> SA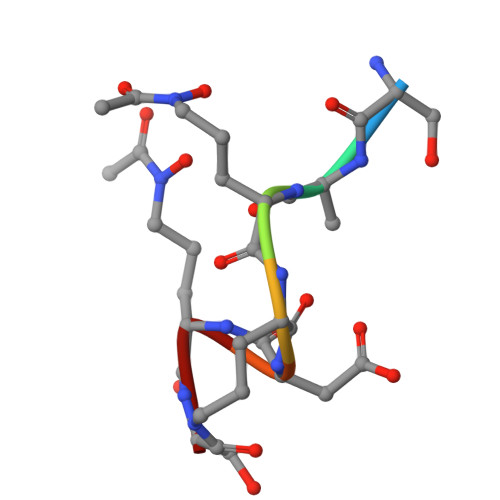AADAS>MCDIGLIGLAVMGQNLSLNISSKGFKIGVYNRTYERTEETMKRAKEENLVVYGYKTVEELINNLKKPRKVILLIKAGPAVDENISNILKHFEKGDIIIDGGNEWYINSERRIKLCKEKDVEYLAMGVSGGEAGARYGCSFMPGGSKYAYDCVKEILEKCSAQVGNSPCVTYIGPGSSGNYVKMVHNGIEYGDMQLISESYVIMKHILKYDNQKLSEVFNKWNEGILNSYLIEITANILAKKDDLTNNYLVDMILDIAGAKGTGKWTMLEATERGIPCPTMCAALDARNISVFKELRTKAESNFNKDNILIDPNEDLNDFENDLLNALYCCKIISYTQGLFLLKQVSEEMNWKLNLGEIARIWRGGCIIRAVFL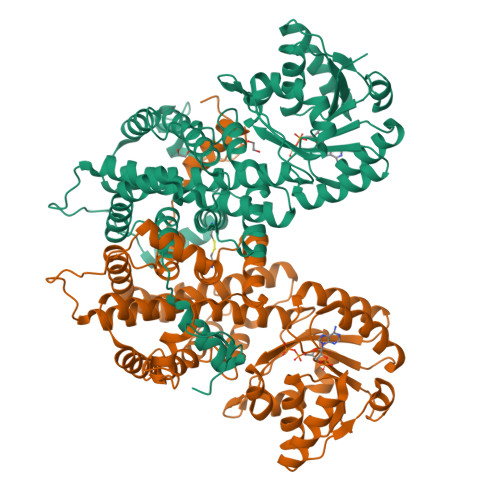DRIANAYKNNEKLELLFLDNEFSDDIKNKLPSLRKIVLMATKYSIPIPAFSASLAYFQMVTSQNLPLNLVQAQRDYFGSHTYRRTDREGNYHTLW[2x]~{N}-[4-(2-chloranylphenoxy)phenyl]-7~{H}-pyrrolo[2,3-d]pyrimidin-4-amine | C18 H13 Cl 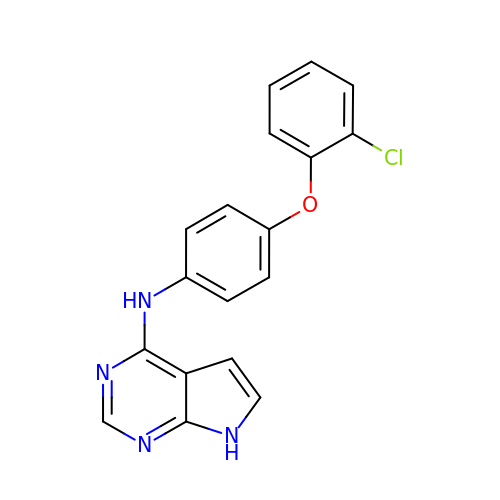N4 O | NHZNMMAEOYALKY-UHFFFAOYSA-N2,3,5-trifluoro-N-hydroxybenzamide | C7 H4 F3 N O2 | 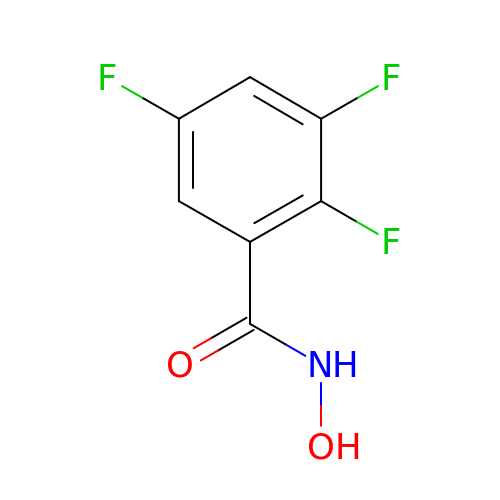KNGFWHCRGOZPON-UHFFFAOYSA-N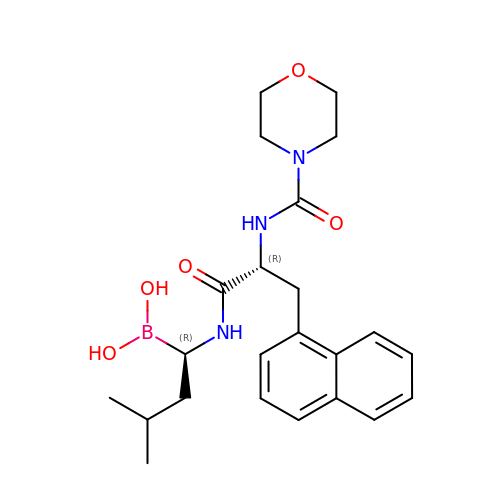(1R)-3-METHYL-1-{[N-(MORPHOLIN-4-YLCARBONYL)-3-(1-NAPHTHYL)-D-ALANYL]AMINO}BUTYLBORONIC ACID | C23 H32 B N3 O5 | MQMHIOPMTAJOHV-RTWAWAEBSA-N> REFTIDFSTQQSYVSSLNSIRTEISTPLEHISQGTTSVSVINHTPPGSYFAVDIRGLDVYQARFDHLRLIIEQNNLAVAGFVNTATNTFYRFSDFTHISVPGVTTVSMTTDSSYTTLQRVAALERSGMQISRHSLVSSYLALMEFSGNTMTRDASRAVLRFVTVTAEALRFRQIQREFRQALSETAPVYTMTPGDVDLTLNWGRISNVLPE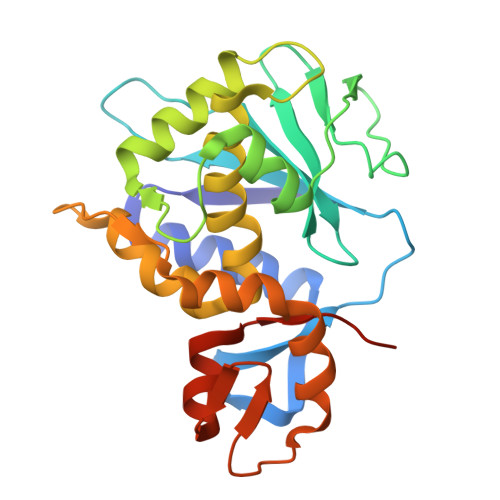YRGEDGVRVGRISFNNISAILGTVAVILNCHHQGARSVR>GGAUUCGUAUAUCCUUAAUGAUAUGGUUUAAGGGCAAUACAUAGAAACCACAAAUUUCUU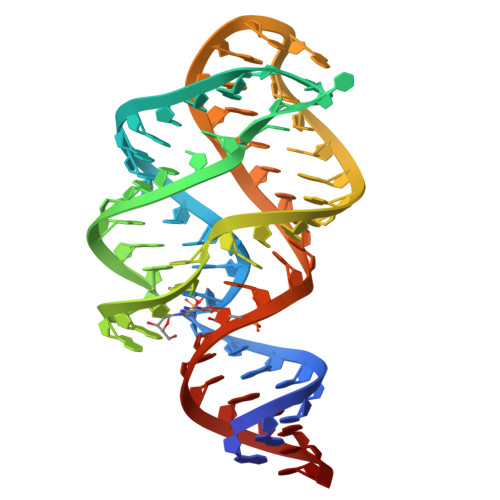ACUGCGAAUUC[2x]> GSIFKPAPHKARLPAAEIDPTYRRLRWQIFLGIFFGYAAYYLVRKNFALAMPYLVEQGFSRGDLGFALSGISIAYGFSKFIMGSVSDRSNPRVFLPAGLILAAAVMLFMGFVPWATSSIAVMFVLLFLCGWFQGMGWPPCGRTMVHWWSQKERGGIVSVWNCAHNVGGGIPPLLFLLGMAWFNDWHAALYMPAFCAILVALFAFAMMRDTPQSCGLPPIEEYKNDYPDDYNEKAEQELTAKQIFMQYVLPNKLLWYIAIANVFVYLLRYGILDWSPTYLKEVKHFALDKSSWAYFLYEYAGIPGTLLCGWMSDKVFRGNRGATGVFFMTLVTIATIVYWMN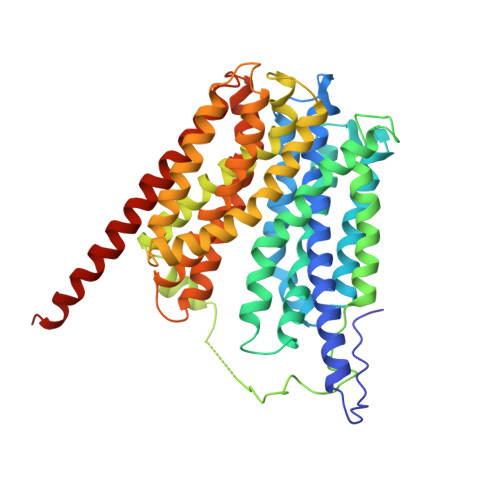PAGNPTVDMICMIVIGFLIYGPVMLIGLHALELAPKKAAGTAAGFTGLFGYLGGSVAASAIVGYTVDFFGWDGGFMVMIGGSILAVILLIVVMIGEKRRHEQLLQELVPR> GSHMNGRIYAVGGYDGNTHLNSVEAYDPETDEWSFVAPMTTPRSGVGVAVLNGRIYAVGGYDGNTHLNSVEAYDPETDEWSFVAPMTTPRSGVG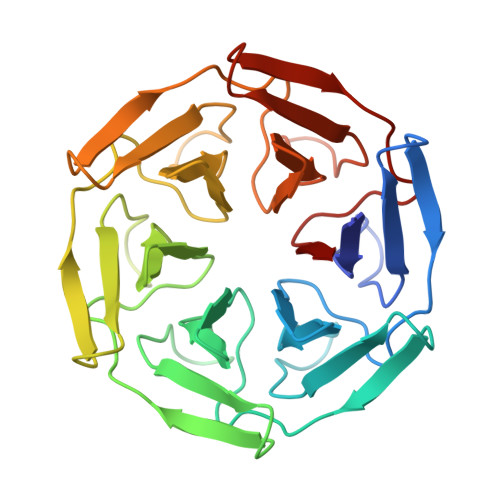VAVLNGRIYAVGGYDGNTHLNSVEAYDPETDEWSFVAPMTTPRSGVGVAVLNGRIYAVGGYDGNTHLNSVEAYDPETDEWSFVAPMTTPRSGVGVAVLNGRIYAVGGYDGNTHLNSVEAYDPETDEWSFVAPMTTPRSGVGVAVLNGRIYAVGGYDGNTHLNSVEAYDPETDEWSFVAPMTTPRSGVGVAVL> MLRARARSAYTVARSSAARCSAAASIGAGSGALNGSTGLGSGVGAGAASASLHEPRRYSFKYATKRQHNEARQPSYIHDKRYGLFSNEHNIGKSRRGLPHITPIYTKHMSLWETDTDASTNRFFRHYVFGQREEHLLLGRPHGFEADQAGGRQGDSAYELNTDQRYKGVPRPAITNLHYEPVWNQTLYRNTAHGNQLTNPSSKLTAAVLGPDLMEVRDIKSVEHCKAWFDRLSFLIQQHYDAVGDIGAFRSRHAQHVHEFFVAFHDALSSFDFQDRYLYDQFAKARPKHLEDLFAIFLEMEANYVNEAYCPRCSLPYATTRYCGEGDPNTPFRKHRGRWAPHQYWGKEWYDVVMRRAEALWYRATEDPFFGTTAHTQRQAEALLSVYVKTKHRAKMVDFLHALRGSKEFLLGQLQITPAMQKAADDLLDSTPHEHLLTNAFKLESSAAKYTGDAQSVPHSPLQMRLDMEMNKYRRQQREEGVVRVPPASWKLDTSAIVPYKVDPQTKHVANWRAVKEGIEQSFLATGLPKEAYTSEEWREMLYLKERIASRGARRAQLEAERQAEEAAMAKKYGQRSPAATSSSSWCVFPDTAWYRVFETAAEALKPYGVTHAGQRVLMRSQTYANPAAVPYTDPVRNASVLLDTTPEACSVFGGFESGEVLRLTPKEPEGAAAFDVVVVGVDKSGAEAEWSLYAMHRDVASQTSKGLLNLGTDCLQLLSSYAKVETTRRRAVLTVLDAQRTLPEEHLGQVVGVRRGELYVQWHLQRGGSSELDRSVAVPLGNPETVKQLYKLQTLTDADGAPALLQEPPSWRTPFRNDFVDERLKELEQAPFKREQWASLIQGKYTPKVKKYGYAQHTTQDDFQTKEYKDRLLARQYFHSPQAFSVIPERHERSVKFMGKWEHQRVCGLPTADRDELEKGWGEAEEISDAAVGAIEQALRDISGRRPGNFVKSPTETQSLRLNESWWTPLEFGWEEHNREQMAFLDSSERSIVEGARLPFGGKRPPFGTTYGMGERISEIAADYAKGFGLGPHGHSPQHDTAHFNTLEAEQQRVKVLGLGNALVRLFHEKLGNQDIQAWSLQQCGESDANVRQLLLSVEEWRTKGRAPSLLLRKVLQRYLKEELDAFNSGLPAHVPRLAVPCADASAADSIGSSSAGCIWVDVDRNAFALEHASQFRRGDSDEPYIVGLVQRAGMSSGSGGALAASPAGSGADNTYAEYIQQDVLQRFEIGLARIVGRGIPSSIIMERTVKNSRGLERESAKMLTLVLVGELAKLLSKMRVTPDNISMVVRGLAQCPEKELLGGGDFAVPVSLIFSWNGPQSNVSAATSNSSSSNANAGASRGAGISAVQQMLERTRHGSSPGSSGSGDGEKMVGKVLEELAWSQDGVAADVLYALQQNKANPTLRQEFLNAFLPVCSNDHQKAQHMYADYTLGKFVPNITVAIEAFVKFLGNISTHPGQLTSDVEYFEVDNARRADGTEGTGQYTQVRLLPPEIGPFQYENTLIESIETAERFRRYGILAGPARVPASGFIAANCKSLTYMTHRDKEVVYVTTENDQGLANALRS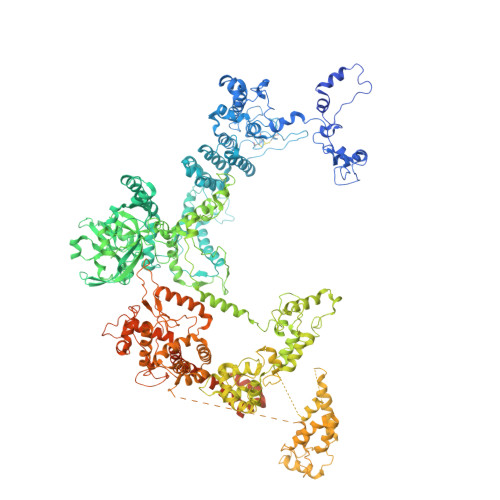SALFKSIASNPKLSYLLKGITGGAPSHPLLVDSFNRFFYRVAPMLSFYQSLLQEYSATMPSAQAEAQIANFGLARALESEASTAIEQDFRRNAERYWRNVLEGRSTEEAALSSGGRESASAQGRRPSQQGSGRAGQSGSGSRRGSGEFNLASVVGHRAAAGARSEKSRVPVSSSSSSSSSTVATAASTSTRVKGLLGSLKGGGSGAGRGKGSRPASPSGVASGSRGGRSSSSNNSGDKNGSTSGRK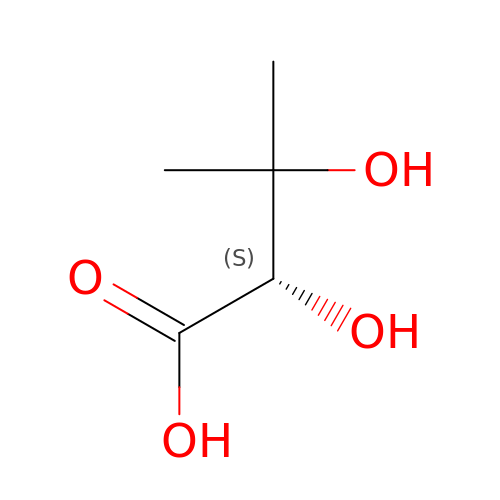(2S)-2,3-dihydroxy-3-methylbutanoic acid | C5 H10 O4 | JTEYKUFKXGDTEU-GSVOUGTGSA-N>[2x]GSHMNYNPEEQFRCTIIRGKAKNMLDNLLPAYANIIDDICPCDKASFVKDFNNRLIEILGEETTKKTLDNHRTEIAGKLFGMFYEDDEVIFPSGRTNKYIEDSDQPAFFKDICFKFQFPNGMDKLDKVIEKVGAKIQIRQFPYI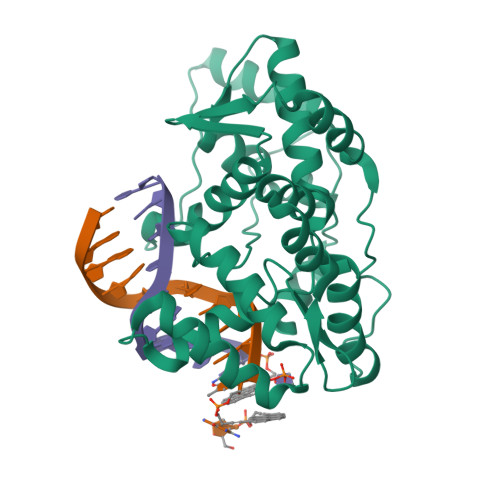LQVLLTADNNNIQLSKDDIAYYVLNSLQVLQGKIKPIEVIEKIIEDRSNDITKKVRHPGKETSYSMQHIREQLNYLELANLIRIDGNLVKLNYREAENINYIAQFWGNKPEFNAYKYDFTSEDDKKSFFKDWQQYYSNVNSHKS> GDRVADVIESSIGDSVSRALTHALPAPTGQNTQVSSHRLDTGKVPALQAAEIGASSNASDESMIETRCVLNSHSTAETTLDSFFSRAGLVGEIDLPLKGTTNPNGYANWDIDITGYAQMRRKVELFTYMRFDAEFTFVACTPTGEVVPQLLQYMFVPPGAPKPDSRESLAWQTATNPSVFVKLSDPPAQVSVPFMSPASAYQWFYDGYPTFGEHKQEKDLEYGAMPNNMMGTFSVRTVGTSKSKYPLVVRIYMRMKHVRAWIPRPMRNQNYLFKANPNYAGNSIKPTGASRTAITTL;> VAQLTIGNSTITTQEAANIIVGYGEWPSYCSDSDATAVDKPTRPDVSVNRFYTLDTKLWEKSSKGWYWKFPDVLTETGVFGQNAQFHYLYRSGFCIHVQCNASKFHQGALLVAVLPEYVIGTVAGGTGTEDTH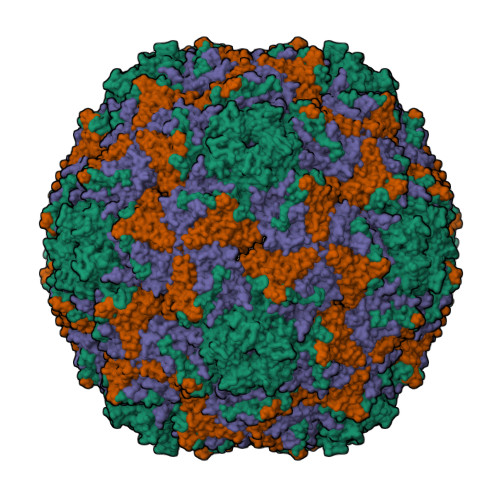PPYKQTQPGADGFELQHPYVLDAGIPISQLTVCPHQWINLRTNNCATIIVPYINALPFDSALNHCNFGLLVVPISPLDYDQGATPVIPITITLAPMCSEFAGLR;> GFPTELKPGTNQFLTTDDGVSAPILPNFHPTPCIHIPGEVRNLLELCQVETILEVNNVPTNATSLMERLRFPVSAQAGKGELCAVFRADPGRNGPWQSTLLGQLCGYYTQWSGSLEVTFMFTGSFMATGKMLIAYTPPGGPLPKDRATAMLGTHVIWDFGLQSSVTLVIPWISNTHYRAHARDGVFDYYTTGLVSIWYQTNYVVPIGAPNTAYIIALAAAQKNFTMKLCKDASDILQTG> MKDYDELLKYYELYETIGTGGFAKVKLACHVLTGEMVAIKIMDKNALGSDLPRVKTEIDALKSLRHQHICQLYHVLETKNKIFMVLEYCPGGELFDYIISQDRLSEEETRVVFRQILSAVAYVHSQGYAHRDLKPENLLFDENHKLKLIDFGLCAKPKGNKDYHLQECCGSLAYAAPELIQGKSYLGSEADVWSMGILLYVLMCGFLPFDDDNVMALYKKIMRGKYEVPKWLSPSSILLLQQMLQVDPKKRISMRNLLNHPWVMQDYSCPVEWQSKTPLTHLDEDCVTELSVH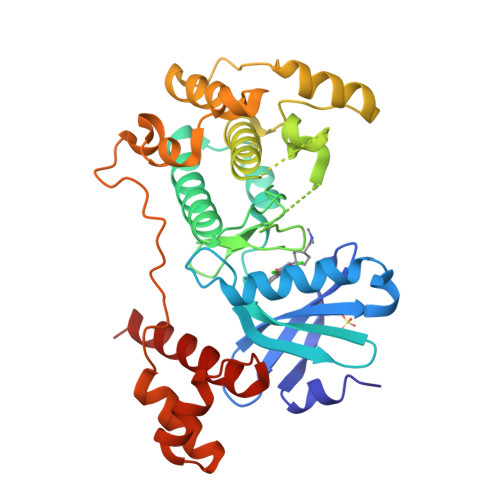HRSSRQTMEDLISSWQYDHLTATYLLLLAKKARLEHHH> MGAQLSLVVQASPSIAIFSYIDVLEEVHYVSQLNSSRFLKTCKALDPNGEIVIKVFIKPKDQYSLRPFLQRIRAQSFKLGQLPHVLNYSKLIETNRAGYMIRQHLKNNLYDRLSLRPYLQDIELKFIAFQLLNALKDIHNLNIVHGDIKTENILVTSWNWCILTDFAAFIKPVYLPEDNPGEFLFYFDTSKRRTCYL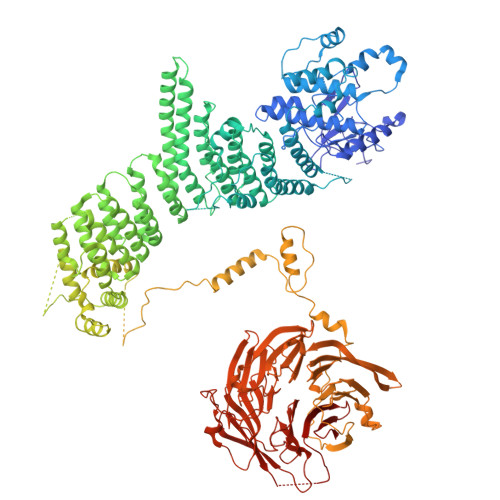APERFNSKLYQDGKSNNGRLTKEMDIFSLGCVIAEIFAEGRPIFNLSQLFKYKSNSYDVNREFLMEEMNSTDLRNLVLDMIQLDPSKRLSCDELLNKYRGIFFPDYFYTFIYDYFRNLVTMTTSTPISDNTCTNSTLEDNVKLLDETTEKIYRDFSQICHCLDFPLIKDGGEIGSDPPILESYKIEIEISRFLNTNLYFPQNYHLVLQQFTKVSEKIKSVKEECALLFISYLSHSIRSIVSTATKLKNLELLAVFAQFVSDENKIDRVVPYFVCCFEDSDQDVQALSLLTLIQVLTSVRKLNQLNENIFVDYLLPRLKRLLISNRQNTNYLRIVFANCLSDLAIIINRFQEFTFAQHCNDNSMDNNTEIMESSTKYSAKLIQSVEDLTVSFLTDNDTYVKMALLQNILPLCKFFGRERTNDIILSHLITYLNDKDPALRVSLIQTISGISILLGTVTLEQYILPLLIQTITDSEELVVISVLQSLKSLFKTGLIRKKYYIDISKTTSPLLLHPNNWIRQFTLMIIIEIINKLSKAEVYCILYPIIRPFFEFDVEFNFKSMISCCKQPVSRSVYNLLCSWSVRASKSLFWKKIITNHVDSFGNNRIEFITKNYSSKNYGFNKRDTKSSSSLKGIKTSSTVYSHDNKEIPLTAEDRNWIDKFHIIGLTEKDIWKIVALRGYVIRTARVMAANPDFPYNNSNYRPLVQNSPPNLNLTNIMPRNIFFDVEFAEESTSEGQDSNLENQQIYKYDESEKDSNKLNINGSKQLSTVMDINGSLIFKNKSIATTTSNLKNVFVQLEPTSYHMHSPNHGLKDNANVKPERKVVVSNSYEGDVESIEKFLSTFKILPPLRDYKEFGPIQEIVRSPNMGNLRGKLIATLMENEPNSITSSAVSPGETPYLITGSDQGVIKIWNLKEIIVGEVYSSSLTYDCSSTVTQITMIPNFDAFAVSSKDGQIIVLKVNHYQQESEVKFLNCECIRKINLKNFGKNEYAVRMRAFVNEEKSLLVALTNLSRVIIFDIRTLERLQIIENSPRHGAVSSICIDEECCVLILGTTRGIIDIWDIRFNVLIRSWSFGDHAPITHVEVCQFYGKNSVIVVGGSSKTFLTIWNFVKGHCQYAFINSDEQPSMEHFLPIEKGLEELNFCGIRSLNALSTISVSNDKILLTDEATSSIVMFSLNELSSSKAVISPSRFSDVFIPTQVTANLTMLLRKMKRTSTHSVDDSLYHHDIINSISTCEVDETPLLVACDNSGLIGIFQ>[2x]MPQDVDFHIPLPGRQSPDHARAEAEQLAWPRSLGLIRSDAAAERHLRGGYADLASRFYPHATGADLDLGVDLMSWYFLFDDLFDGPRGENPEDTKQLTDQVAAALDGPLPDTAPPIAHGFADIWRRTCEGMTPAWCARSARHWRNYFDGYVDEAESRFWNAPCDSAAQYLAMRRHTI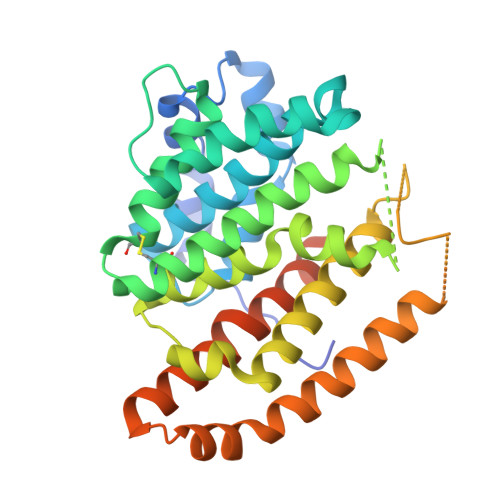GVQPTVDLAERAGRFEVPHRVFDSAVMSAMLQIAVDVNLLLNDIASLEKEEARGEQNNMVMILRREHGWSKSRSVSHMQNEVRARLEQYLLLESCLPKVGEIYQLDTAEREALERYRTDAVRTVIRGSYDWHRSSGRYDAEFALAAGAQGYLEELGSSAH>GPDEEPEEPGRRGSFVEMVDNLRGKSGQGYYVEMTVGSPPQTLNILVDTGSSNFAVGAAPHPFLHRYYQRQLSSTYRDLRKGVYVPYTQGKWEGELGTDLVSIPHGPNVTVRANIAAITE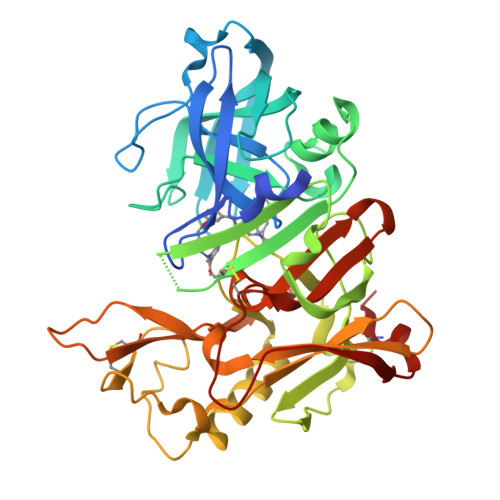SDKFFINGSNWEGILGLAYAEIARPDDSLEPFFDSLVKQTHVPNLFSLQLCGAGFPLNQSEVLASVGGSMIIGGIDHSLYTGSLWYTPIRREWYYEVIIVRVEINGQDLKMDCKEYNYDKSIVDSGTTNLRLPKKVFEAAVKSIKAASSTEKFPDGFWLGEQLVCWQAGTTPWNIFPVISLYLMGEVTNQSFRITILPQQYLRPVEDVATSQDDCYKFAISQSSTGTVMGAVIMEGFYVVFDRARKRIGFAVSACHVHDEFRTAAVEGPFVTLDMEDCGYNI[3x]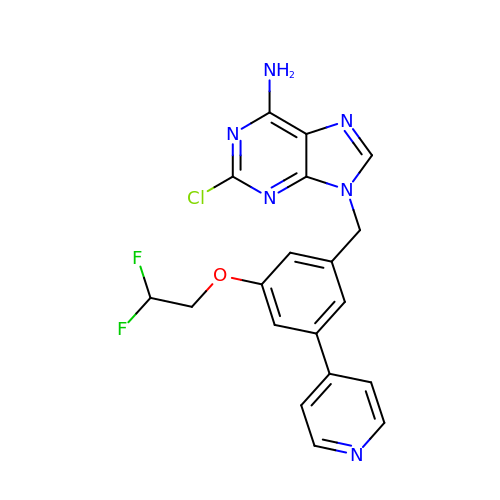2-chloro-9-(3-(2,2-difluoroethoxy)-5-(pyridin-4-yl)benzyl)-9H-purin-6-amine | C19 H15 Cl F2 N6 O | WQJJOKCRYDFRJI-UHFFFAOYSA-N>[3x]MRLAPLYRNALLLTGLLLSGIAAVQAADWPRQITDSRGTHTLESQPQRIVSTSVTLTGSLLAIDAPVIASGATTPNNRVADDQGFLRQWSKVAKERKLQRLYIGEPSAEAVAAQMPDLILISATGGDSALALYDQLSTIAPTLIINYDDKSWQSLLTQLGEITGHEKQAAERIAQFDKQLAAAKEQIKLPPQ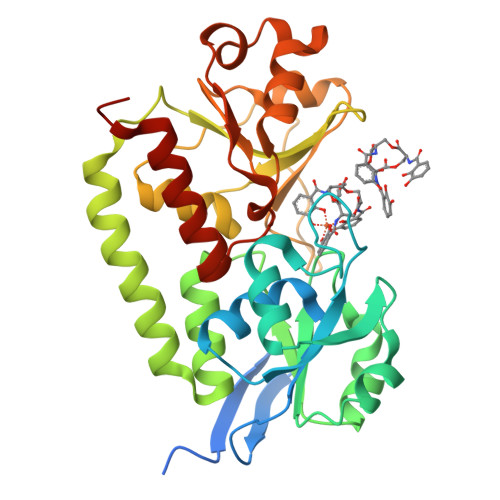PVTAIVYTAAAHSANLWTPESAQGQMLEQLGFTLAKLPAGLNASQSQGKRHDIIQLGGENLAAGLNGESLFLFAGDQKDADAIYANPLLAHLPAVQNKQVYALGTETFRLDYYSAMQVLDRLKALFLEHHHHHH> METIKSIADMATGVVSSVDSTINAVNEKVESVGNEIG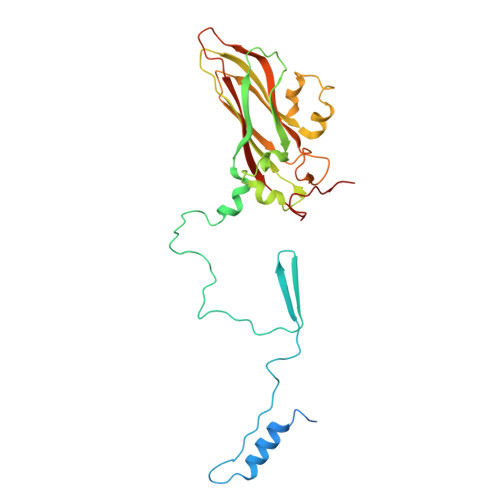GNLLTKVADDASNILGPNCFATTAEPENKNVVQATTTVNTTNLTQHPSAPTMPFSPDFSNVDNFHSMAYDITTGDKNPSKLVRLETHEWTPSWARGYQITHVELPKVFWDHQDKPAYGQSRYFAAVRCGFHFQVQVNVNQGTAGSALVVYEPKPVVTYDSKLEFGAFTNLPHVLMNLAETTQADLCIPYVADTNYVKTDSSDLGQLKVYVWTPLSIPTGSANQVDVTILGSLLQLDFQNPRVFAQDVNIYDN The pneumococcal serine-rich repeat protein (PsrP) is an important lung-specific virulence factor that is present in 60% of strains capable of causing pneumonia in children. Pneumococcal PsrP promotes both biofilm formation through self-oligomerization and adherence to keratin 10 (KRT10)-expressing lung epithelial cells. In this study, the crystal structure of the KRT10-binding region of PsrP (BR187–385) was determined, revealing a novel fold distantly related to CnaA subdomains. While one face of the compressed, two-sided barrel of BR187–385 is created by an extended β-sheet that presents a highly basic binding groove, extensive well-ordered loop regions distort the other face of the barrel, forming a paperclip-like substructure.

BR187–385 crystallized in two crystal forms of the space groups P43212 and P4122, with differing unit cell parameters. Single anomalous dispersion (SAD) data, collected from a seleno-methionine derivative of the P43212 crystal form that diffracted to 2.25 Å, was used to solve the phase problem. Three BR187–385 polypeptide chains were placed in the asymmetric unit, and refined to R- and Rfree-values of 18.6% and 21.5%, respectively. The structural deviation between the P4122-BR187–385 monomer and each of the three P43212-BR187–385 molecules was minimal, with root mean square deviations (r.m.s.d.) of 0.6 Å and less than 0.4 Å, following superposition of the P4122 monomer on the P43212 chains A and B/C, respectively. Crystal packing analysis revealed that two symmetry-related molecules in the P4122 crystal formed an intermolecular β-sheet resulting in an interface area of 585 Å2. The same interface was also observed for chains B and C in the P43212 crystal form. We believe, at the present stage, that the formed pseudo-complexes are probably owing to crystal packing. In conclusion, the crystal structure of the BR187–385 monomer takes a compressed barrel fold with one face formed by an extended and twisted β-sheet, and the other face mainly consisting of well-ordered loops.

>[3x]HHHHHHSGNTIVNGAPAINASLNIAKSETKVYTGEGVDSVYRVPIYYKLKVTNDGSKLTFTYTVTYVNPKTNDLGNISSMRPGYSIYNSGTSTQTMLTLGSDLGKPSGVKNYITDKNGRQVLSYNTSTMTTQGSGYTWGNGAQMNGFFAKKGYGLTSSWTVPITGTDTSFTFTPYAARTDRIGINYFNGGGKVVESSTTSQSLSQ> MQSNKTFNLEKQNHTPRKHHQHHHQQHHQQQQQQQQQPPPPIPANGQQASSQ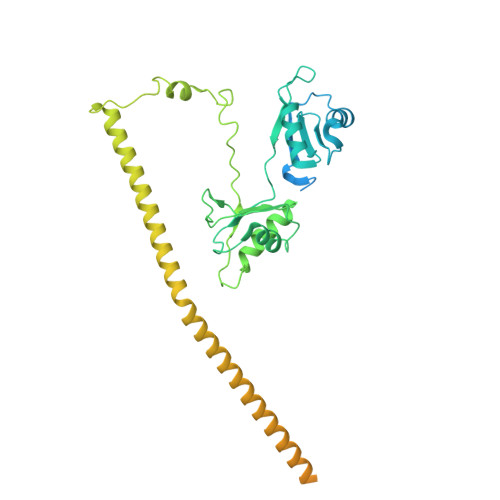NEGLTIDLKNFRKPGEKTFTQRSRLFVGNLPPDITEEEMRKLFEKYGKAGEVFIHKDKGFGFIRLETRTLAEIAKVELDNMPLRGKQLRVRFACHSASLTVRNLPQYVSNELLEEAFSVFGQVERAVVIVDDRGRPSGKGIVEFSGKPAARKALDRCSEGSFLLTTFPRPVTVEPMDQLDDEEGLPEKLVIKNQQFHKEREQPPRFAQPGSFEYEYAMRWKALIEMEKQQQDQVDRNIKEAREKLEMEMEAARHEHQVMLMRQDLMRRQEELRRMEELHNQEVQKRKQLELRQEEERRRREEEMRRQQEEMMRRQQEGFKGTFPDAREQEIRMGQMAMGGAMGINNRGAMPPAPVPTGTPAPPGPATMMPDGTLGLTPPTTERFGQAATMEGIGAIGGTPPAFNRPAPGADFAPNKRRRY> ATFEIVNRCSYTVWAAASKGDAALDAGGRQLNSGESWTINVEPGTNGGKIWARTDCYFDDSGSGICKTGDCGGLLRCKRFGRPPTTLAEFSLNQYGKDYIDISNIKGFNVPMNFSPTTRGCRGVRCAADIVGQCPAKLKAPGGGCNDACTVFQTSEYCCTTGKCGPTEYSRFFKRLCPDAFSYVLDKPTTVTCPGSSNYRVTFCPT

Here, a series of new methods are presented based on the use of a low X-ray-background film as a crystallization support and a photoablation laser that enable the automation of major operations required for the preparation of crystals for X-ray diffraction experiments. In this approach, the controlled removal of the mother liquor before crystal mounting simplifies the cryocooling process, in many cases eliminating the use of cryoprotectant agents, while crystal-soaking experiments are performed through diffusion, precluding the need for repeated sample-recovery and transfer operations. We have previously shown that the transfer of crystals to X-ray data-collection pins can be automated through the so-called CrystalDirect approach, which relies on the use of a thin, low X-ray-background film as a crystallization support from which crystals are recovered by excising the film with a laser beam and attaching it to an X-ray data-collection pin. The CrystalDirect system enables the automation of sample mounting and cryocooling and can contribute to closing the automation gap that currently exists between crystallization and X-ray data collection.

As an initial validation, crystals of proteinase K, thaumatin and lysozyme were prepared in CrystalDirect plates. These crystals grow from solutions that typically require the addition of cryoprotectants when mounted manually. Femtosecond photoablation lasers, such as that used here, produce little or no collateral damage to the sample owing to heat conduction or shock waves. A series of ablation experiments performed on thaumatin crystals confirmed that the effects of ablation do not propagate through the crystal.> SNAIPIFLSVLQSIEPEVVYAGYDNTQPDTSASLLTSLNELGERQLVRVVKWAKALPGFRNLHVDDQMTLIQYSWMGVMVFAMGWRSYKNVNSRMLYFAPDLVFNEQRMQKSTMYNLC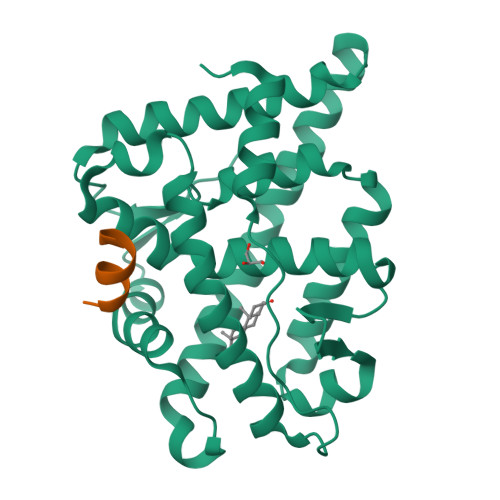VRMRHLSQEFVWLQVTQEEFLCMKALLLFSIIPVEGLKNQKYFDELRMNYIKELDRVISFQGKNPTSSSQRFYQLTKLLDSLQPIVRKLHQFTFDLFVQSQSLSVEFPEMMSEIISAQVPKILAGMVKPLLFHKQ;> QALLRYLLDKDD>[7x]MTKINWEKYKKVIKKEFSEKEETEEVKNYIFSSQLDKVNLILEHMDTVGGIHSRNIAITGDRGTGKTSFIETLKLVLEKQNYYVFDIVSPTVLSSHLNILEIVISSIYREIDQFIDSHDVHDRGRLIQHLKKVMNAIAVEKKQSDYFKQSKPEIEMLTDLSHRTFLDEEIKELFCYFKKVLNNRQDSCKEVIKDLVLIIDDLDLVENNLVYDLLRDIQHYLDSQLIVIFAYKEGQLEQSMFEHLAKGNEALLNHGVIDSNAIFGQIERFLTKLVPLSNRIPLFKQDELLNKTIGEFLASLDPSYGVGENLEFITKDSEKNKNNLTIREWFYESIFYRTNLKLDPIDIREEASRLMPKTLREMVQLCEELHSMQVITRSMDKLAGVEGLRKNIGAFRRYIGYKNSTYFNLATMEFFQKWELAESHQANYLAYHFLMSYYQESFEQNQKLGYPLNLSKSGYPLTLRTMEPYNITLGDIYALMEELKYTEGISADTYYIVYILKVYYSLRLSELLYNVVLHHKLFVHVKEEATTFYMATSTEELQIEKNHEQEATKLTDKEYREHIMTAIEKVPALQAYLELVNAQFMPQNFNYDRSGSRDDDFYLISWLKDDDLPEYSRLFKSLFLNSEVAAKGQIQRNIGKRESVFRYRNLYSYLPLQLTSATFYKIDFLAFAIKADLLMYNVVRFVEEEGDTIPYFMSNMFHIDVFVRHNYNENNNKGKFAYIAKQIVFGLWQGSNQRAHDLKHWYKSFDTVFGTKIEALHLLVDIAEQIKISDKQTTDVSALSEEQKRDEQAKKVAEKLAAIYHHIGMSRILSRLHQLPFIAEIKSNKELLQHFSEAIVKLEKYASDTINVGNLSQFRESLKKIGQTYPSIQVLVDKLHRKQKLYVEFIQDFIETVNKLGEADESN

The RADAR system comprises two genes, rdrA that encodes a protein with an ATPase domain, and rdrB, encoding a predicted adenosine deaminase domain protein. Here, we determine cryo-EM structures of the RADAR defense complex, revealing RdrA as a heptameric, two-layered AAA+ ATPase and RdrB as a dodecameric, hollow complex with twelve surface-exposed deaminase active sites. RdrA and RdrB join to form a giant assembly up to 10 MDa, with RdrA docked as a funnel over the RdrB active site. Our results define ATP mononucleotide deamination as a determinant of RADAR immunity and reveal supramolecular assembly of a nucleotide-modifying machine as a mechanism of anti-phage defense.

To better understand the RdrA C-terminal domain, we next determined a 2.5 Å cryo-EM structure of the divergent (<20% amino acid identity) RdrA from Streptococcus suis. S. suis RdrA adopts a similar two-layered heptameric architecture confirming conservation of the C-terminal α-helical lobe despite high sequence variability. Interestingly, S. suis RdrA particles existed primarily as 14-mer complexes with the RdrA stacked head-to-tail. In this conformation, although the ATPase domains are highly similar (RMSD 2.7 Å), the final four α helices of the RdrA C terminus undergo a dramatic ∼120° reorientation relative to the E. coli RdrA structure and flip out to form a protein-protein binding interface.> GSAKDVKFGADARALMLQGVDLLADAVAVTMGPKGRTVIIEQSWGSPKVTKDGVTVAKSIDLKDKYKNIGAKLVQDVANNTNEEAGDGTTTATVLARSIAKEGFEKISKGANPVEIRRGVMLAVDAVIAELKKQSKPVTTPEEIAQVATISANGDKEIGNIISDAMKKVGRKGVITVKDGKTLNDELEIIEGMKF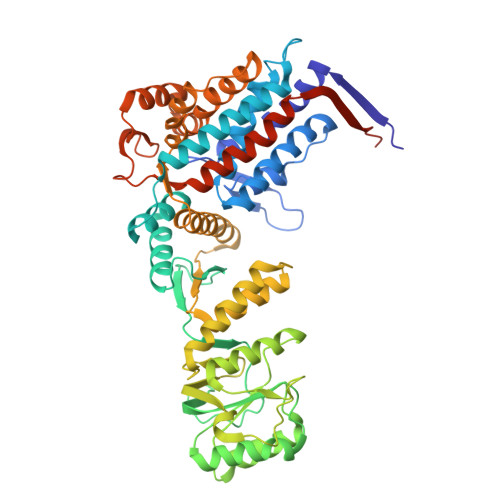DRGYISPYFINTSKGQKCEFQDAYVLLSEKKISSIQSIVPALEIANAHRKPLVIIAEDVDGEALSTLVLNRLKVGLQVVAVKAPGFGDNRKNQLKDMAIATGGAVFGEEGLTLNLEDVQPHDLGKVGEVIVTKDDAMLLKGKGDKAQIEKRIQEIIEQLDVTTSEYEKEKLNERLAKLSDGVAVLKVGGTSDVEVNEKKDRVTDALNATRAAVEEGIVLGGGCALLRCIPALDSLTPANEDQKIGIEIIKRTLKIPAMTIAKNAGVEGSLIVEKIMQSSSEVGYDAMAGDFVNMVEKGIIDPTKVVRTALLDAAGVASLLTTAEVVVTEIPKEEKDPGMGAMGGMGGGMGGGMF> GPGSKPQEPATAEIKPNKKILIELKVEKKPMGVIVCGGKNNHVTTGCVITHVYPEGQVAADKRLKIFDHICDINGTPIHVGSMTTLKVHQLFHTTYEKAVTLTVFRADPPELEKFNVDLMKKAGKELGLSLSPNEIGCTIADLIQGQYPEIDSKLQRG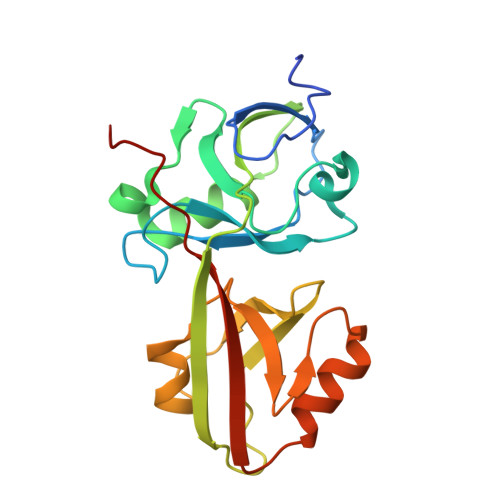DIITKFNGDALEGLPFQVCYALFKGANGKVSMEVTRPKPTLRTEAPKA>[3x]GPHMPGSGQIQ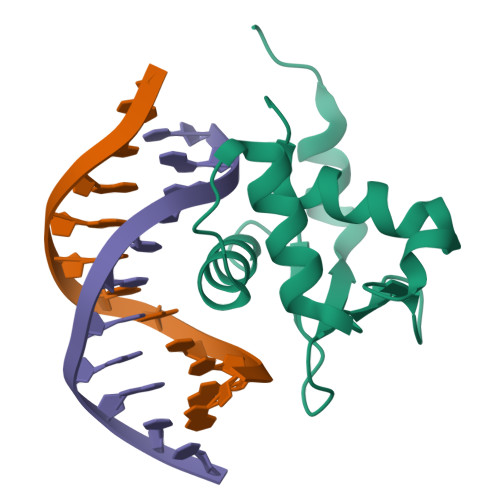LWQFLLELLSDSANASCITWEGTNGEFKMTDPDEVARRWGERKSKPNMNYDKLSRALRYYYDKNIMTKVHGKRYAYKFDFHGIAQALQPHPTE5-[(2~{S},7~{R})-7-chloranyl-2-methyl-octyl]benzene-1,3-diol 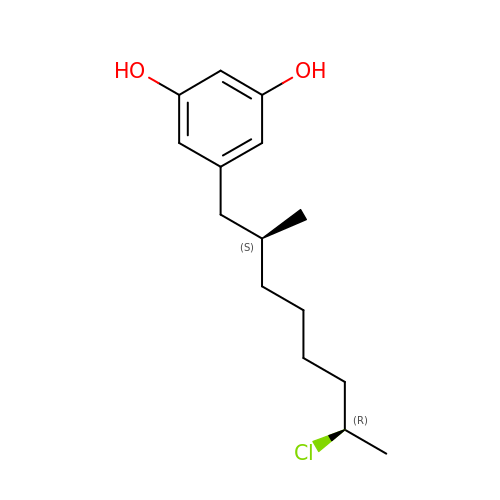| C15 H23 Cl O2 | IDGYFUOTKOBQGZ-NWDGAFQWSA-N> SNATGFLVSFMVDARGGSMRGSRHNGLRVVIPPRTCAAPTRITCRLVK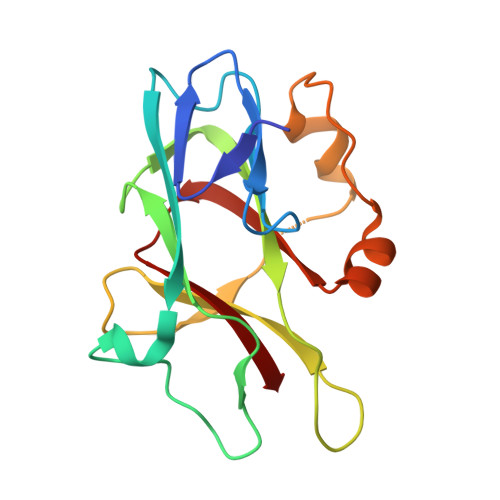PQKLSTPPPLAEEEGLASRIIALGPTGAQFLSPVIVEIPHFASHGRGDRELVVLRSENGSVWKEHRSRYGESYLDQILNGMDEELGSLEELEKKRVCRIITTDFPLYFVIMSR> KK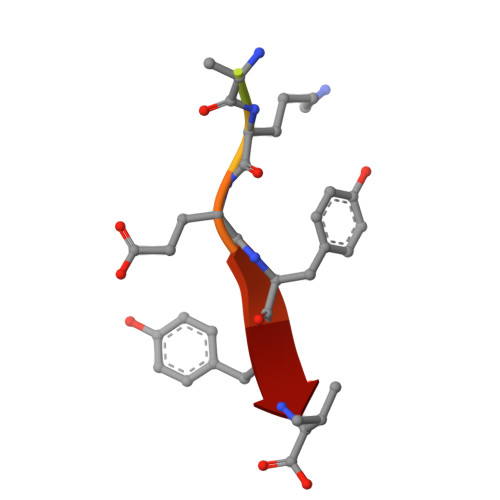NKDKEYYV> MGHHHHHHMFLRNSVLRTAPVLRRGITTLTPVSTKLAPPAAASYSQAMKANNFVYVSGQIPYTPDNKPVQGSISEKAEQVFQNVKNILAESNSSLDNIVKVNVFLADMKN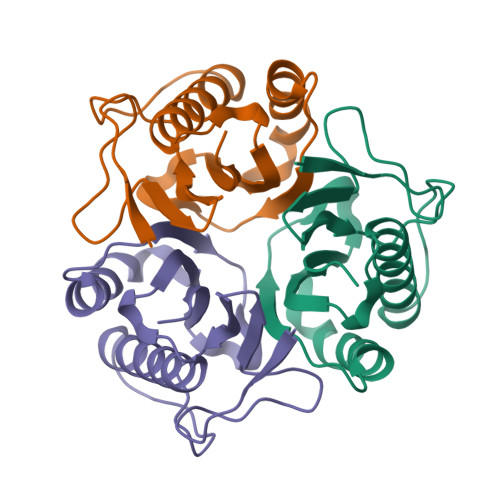FAEFNSVYAKHFHTHKPARSCVGVASLPLNVDLEMEVIAVEKN>GAAQPAMAQGALLQAQALYPWRAKKDNHLNFNKNDVITVLEQQDMWWFGEVQGQKGWFPKSYVKLISAAA[2x];>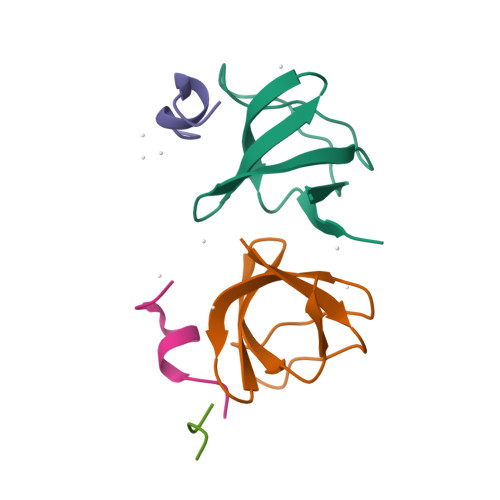WRDSSGYVMGPW[3x]>[2x]MGSSHHHHHHSSGLVPRGSHMASAASYPPIKNTKVGLALSSHPLASEIGQKVLEEGGNAIDAAVAIGFALAVVHPAAGNIGGGGFAVIHLANGENVALDFRE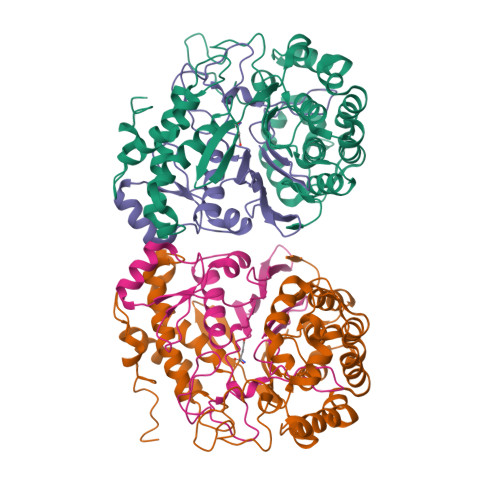KAPLKATKNMFLDKQGNVVPKLSEDGYLAAGVPGTVAGMEAMLKKYGTKKLSQLIDPAIKLAENGYAISQRQAETLKEARERFLKYSSSKKYFFKKGHLDYQEGDLFVQKDLAKTLNQIKTLGAKGFYQGQVAELIEKDMKKNGGIITKEDLASYNVKWRKPVVGSYRGYKIISMSPPSSGGTHLIQILNVMENADLSALGYGASKNIHIAAEAMRQAYADRSVYMGDADFVSVPVDKLINKAYAKKIFDTIQPDTVTPSSQIKPGMGQLHEGSN;>TTHYSVADRWGNAVSVTYTINASYGSAASIDGAGFLLNNEMDDFSIKPGNPNLYGLVGGDANAIEANKRPLSSMSPTIVLKNNKVFLVVGSPGGSRIITTVLQVISNVIDYNMNISEAVSAPRFHMQWLPDELRIEKFGMPADVKDNLTKMGYQIVTKPVMGDVNAIQVLPKTKGSVFYGSTDPRKEF[2x]>MTPSHPARPSRSGILVFDVNETLLDLTSLSPLFERVFGDAKVLREWFPELILYSQTLTLTGLYRPFGEIAAAVFEMVAANHQAKVTPDDIAELKTRLTSMPAYPDVAPALTRLQDAGFRLVTLTNSAPSPAPSPLEKAGIASFFEAHLTVHSSQRFKPHPSVYDSTAETLGAKPEELCMIACNIWDTIGAQARGWRGGFVARPH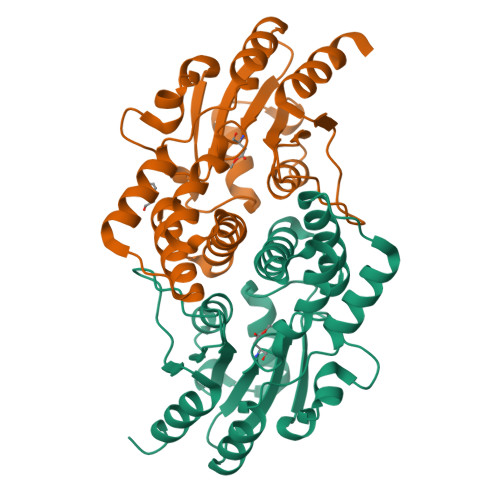NTPLTLAEVPQPDFIGRDMGELADQLIASLTA[2x]>S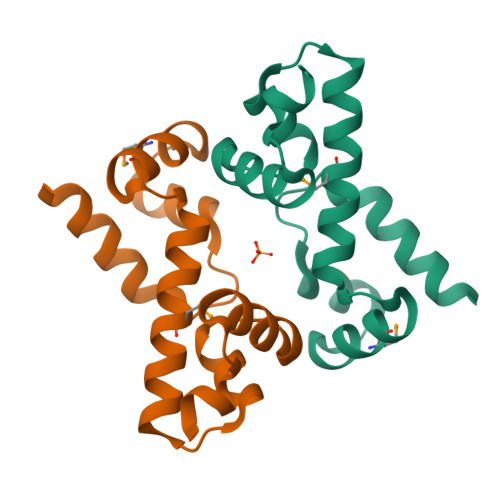NAKELIQNIIEESYTDSQFTLSVLSEKLDLSSGYLSIMFKKNFGIPFQDYLLQKRMEKAKLLLLTTELKNYEIAEQVGFEDVNYFITKFKKYYQITPKQYRE[5x]> MKSLSFMRVLEAVRTMLQEKGGLDVSIVMRNQVEMPTTMIEMIDQEEEESQTAWKEKYRFAIHHYTNEQDLAGVEKIDTLIQMGFILPEGYKLVAVRHCGKQNLVKENTLIHAKTS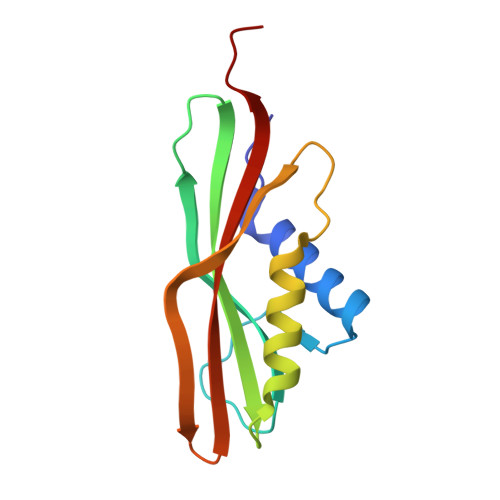FEVSICRELKVKI> TPLGPASSLPQSFLLKCLEQVRKIQGDGAA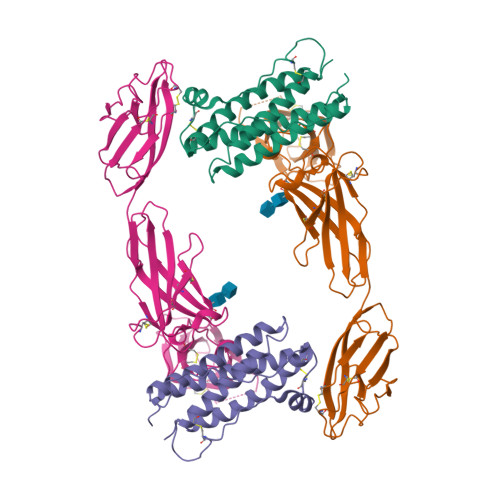LQEKLCATYKLCHPEELVLLGHSLGIPWAPLSSCPSQALQLAGCLSQLHSGLFLYQGLLQALEGISPELGPTLDTLQLDVADFATTIWQQMEELGMAPALQPTQGAMPAFASAFQRRAGGVLVASHLQSFLEVSYRVLRHLAQP;> ECGHISVSAPIVHLGDPITASCIIKQNCSHLDPEPQILWRLGAELQPGGRQQRLSDGTQESIITLPHLNHTQAFLSCSLNWGNSLQILDQVELRAGYPPAIPHNLSCLMNLTTSSLICQWEPGPETHLPTSFTLKSFKSRGNCQTQGDSILDCVPKDGQSHCSIPRKHLLLYQNMGIWVQAENALGTSMSPQLCLDPMDVVKLEPPMLRTMDPSPEAAPPQAGCLQLSWEPWQPGLHINQKCELRHKPQRGEASWALVGPLPLEALQYELCGLLPATAYTLQIRCIRWPLPGHWSDWSPSLELRTTERAAAPR>[2x]EPKLDMNKQKISPAEVAKHNKPDDCWVVINGYVYDLTRFLPNHPGGQDVIKFNAGKDVTAIFEPLHAPNVIDKYIAPEKKLGPLQGSMPPELVCPPYAPGETKEDIARKEQLKSLLPPLDNIINLYDFEYLASQTLTKQAWAYYSSGANDEVTHRENHNAYHRIFFKPKILVDVRKVDISTDMLGSHVDVPFYVSATALCKLGNPLEGEKDVA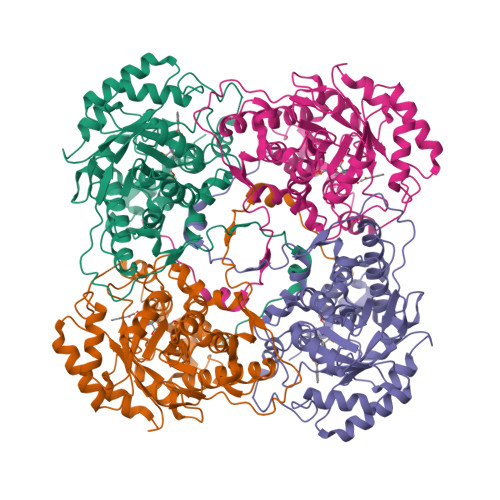RGCGQGVTKVPQMISTAASCSPEEIIEAAPSDKQIQWYQLYVNSDRKITDDLVKNVEKLGVKALFVTVDAPSLGQREKDMKLKFSNTKAGPKAMKKTNVEESQGASRALSKFIDPSLTWKDIEELKKKTKLPIVIKGVQRTEDVIKAAEIGVSGVVLSNHGGRQLDFSRAPIEVLAETMPILEQRNLKDKLEVFVDGGVRRGTDVLKALCLGAKGVGLGRPFLYANSCYGRNGVEKAIEILRDEIEMSMRLLGVTSIAELKPDLLDLSTLKARTVGVPNDVLYNEVYEGPTLTEFEDA>APVNTTTEDETAQIPAEAVIGYSDLEGDFDVAVLPFSNSTNNGLLFINTTIASIAAKEEGVSLEKREAEAEFQSKDGVEDLDGPGDDLYVKDLSGCPGYKATKHWQTRSGFYADLTLAGPACNVFGTDLPDLKLEVEYQTSDRLHVKILDTNNTVYQVPDSVFPRPGFGEWCSPKDSKLKFDFQADPFSFTVSRTDTGEVLFDTTGNKLVFESQYVYLKTHLPQNPHLYGLGEHSDAFMLNTTNYTRTIYTRDAYGTPQGENLYGAHPIYFDHRQTGTHGVFLLNSNGMDIFIDNNATQYLEYNIIGGVLDFYFIAGPSPRDVAIQYAEITQTPLMTPYWGLGYHQCKYGYQDVYEVAAVVANYSTNNIPLETIWTDIDYMDRRRIFTIDPERFPANLYKDLVDTIHARDQHYIVMVDPAVYYKESNPALDEGLRYDIFMKENNGSEYQGVVWAGPSHFPDWFHPDSQQYWSEQFLAFFDGTNGPDIDALWIDMNEPANFYNRPYPGNNTTPENFAEVDGDPPAAPAVRDGPDAPIPGFPASLQPNWV[8x];>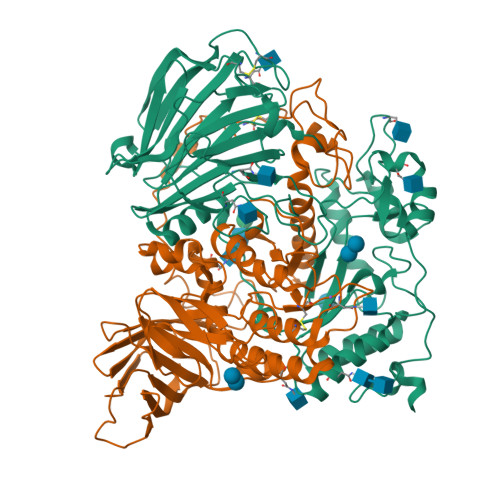[8x]SRRNLGAGHWKSPKGKVDPRAGWQNGKQTGSGCGPNECKGLPNRHLIRPPYMIQNGAGPTLADSTADTDLVQSGGYVQYDTHNLYGAMMSSHSHNAMRARRPDDRALVITRSTFAGSGKDVSHWLGDNVSGWLWYQLSISQILQFASLYQIPVVGPDVCGFGGNVTETLCARWATLGSFYTFFRNHAEIYANPQEFYRWPTVAQAARNGISIRYQLLDYIYTAIYKQNQTGTPALNPLFFNYPNDPNTYPIDLQFFYGDGILVSPVTEENSTSVTFYLPDDIFYEWGTGKPVRGQGEYVSLDNIDYTDITIHYKGGIVYPQRIESANTTTALRQKGFNIVVAPGLDGRAEGSLYLDDGVSVVQDTVSEIDFVYENGKLTMTGSFEYEAGVGIETITVLGVESKPEGDEDVEYDAENKKLVKHVDVPLTGENEITILAVDHHHHHH> DEVLFTGVKEVDDFFEQEKNFLINYYNRIKDSCVKADKMTRSHKNVADDYIHTAACLHSLALEEPTVIKKYLLKVAELFEKLRKVEGRVSSDEDLKLTEL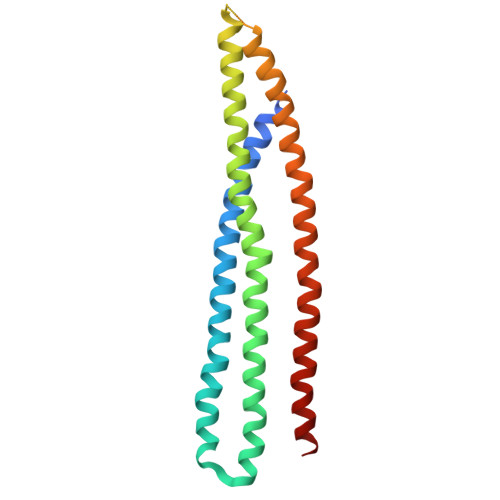LRYYMLNIEAAKDLLYRRTKALIDYENSNKALDKARLKSKDVKLAEAHQQECCQKFEQLSESAKEELINFKRKRVAAFRKNLIEMSELEIKHARNNVSLLQSCIDLFKNN> 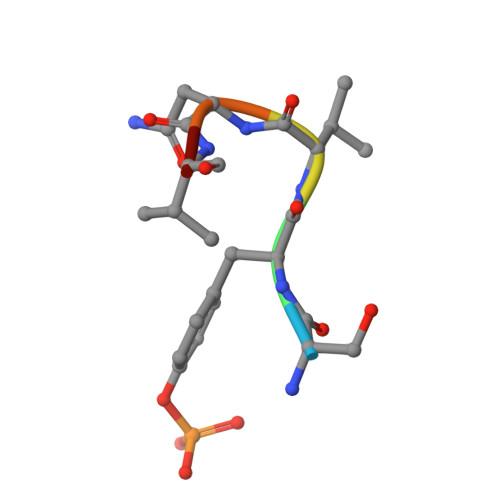SYVNVQ>[4x]MVGLIWAQATSGVIGRGGDIPWRLPEDQAHFREITMGHTIVMGRRTWDSLPAKVRPLPGRRNVVLSRQADFMASGAEVVGSLEEALTSPETWVIGGG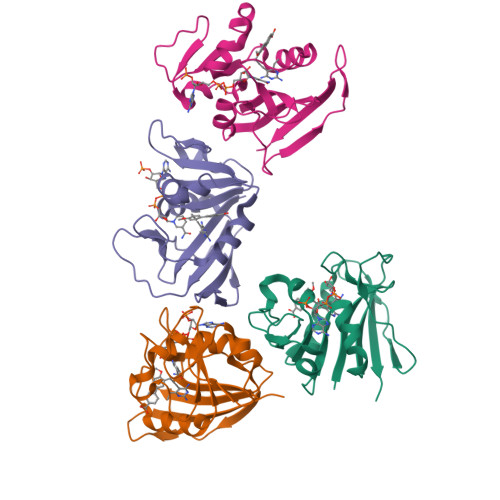QVYALALPYATRCEVTEVDIGLPREAGDALAPVLDETWRGETGEWRFSRSGLRYRLYSYHRS>[13x]MTIDINKLKEELGLGDLAKSLEGLTAAQKAQEAERMRKEQEEKELARMNALVSKAVGEDRQKLEQALELVKS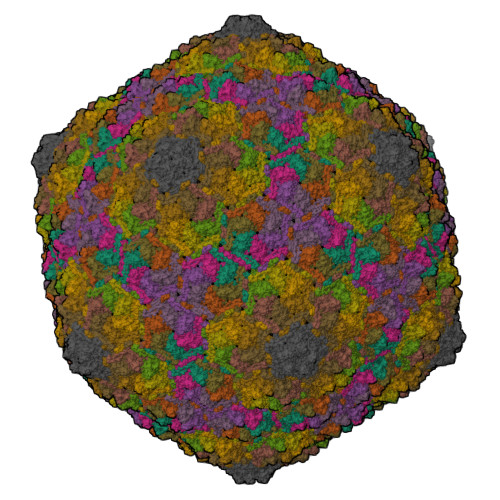LDEKSKKSAELFAQTVEKQQETIVGLQDEIKSLLTAREGRSFVGDSVAKALYGTQETFEDEVEKLVLLSYVMEKGVFETEHGQKHLKAVNQSSSVEVSSESYETIFSQRIIRDLQKELVVGALFEELPMSSKILTMLVEPDAGRATWVAASAYGSDNTTGSEVTGALTEIHFSTYKLAAKSFITDETEEDAIFSLLPLLRKRLIEAHAVSIEEAFMTGDGSGKPKGLLTLASEDSAKVTTEAKADGSVLVTAKTISKLRRKLGRHGLKLSKLVLIVSMDAYYDLLEDEEWQDVAQVGNDAVKLQGQVGRIYGLPVVVSEYFPAKAAGKEFAVIVYKDNFVMPRQRAVTVERERQAGKQRDAYYVTQRVNLQRYFENGVVSGAYAAS Pyruvate decarboxylase (PDC; EC 4.1.1.1) catalyses the non-oxidative decarboxylation of pyruvate to acetaldehyde with the release of carbon dioxide, and is a key enzyme in homofermentative metabolism, where ethanol is the main fermentation product. ZpPDC forms a tetramer from four identical subunits in a dimer-of-dimers fashion. Each monomer contains a pyrimidine-binding (PYR) domain, a regulatory (R) domain and a pyrophosphate-binding (PP) domain. The TPP molecules bind across both subunits in each dimer, with the pyrophosphate group binding to the PP domain from one subunit and the pyrimidine ring binding to the PYR domain from the second subunit, thus forming two active sites in the dimer.

In this study, we present the crystal structure of recombinant ZpPDC at 2.15 Å resolution together with a comparison to the other known bacterial PDCs, thereby increasing the structural information available on these rare enzymes. The final model contains six tetramers in the asymmetric unit, each with a surface area of 65 000 Å2. It comprises 24 amino-acid chains of 555 amino acids, each with a TPP and a Mg2+ ion, and 4147 water molecules. Despite crystallization in the presence of pyruvate, no pyruvate molecules were visible anywhere in the structure, probably owing to catalytic turnover of the substrate to acetaldehyde and subsequent loss of this volatile product. However, six 1,2-ethanediol (EDO) molecules (the PEG monomer) are present, four of which can be found in the active sites in chains I, N, Q and R. Through pseudo-222 symmetry, the four monomers in a tetramer create four cofactor- and substrate-binding sites located in narrow clefts on the interfaces between the PYR domain of one monomer and the PP domain of a second monomer. The TPP molecule binds as indicated by the domain nomenclature, with the pyrophosphate group binding to the PP domain of one monomer and the pyrimidine ring binding to the PYR domain of a second monomer in the dimer. The pyrophosphate group of TPP is anchored to the protein by a Mg2+ ion. It forms an octahedral coordination sphere with the two O atoms on the diphosphate group of the TPP, the side-chain O atoms of Asp435 and Asn462, the main-chain O atom of Gly464 and a water molecule. Glu468 and Tyr289 from one monomer and Asp26, His112 and His113 from a second monomer interact with EDO through an extensive hydrogen-bond network.

>MYTVGMYLAERLAQIGLKHHFAVAGDYNLVLLDQLLLNKDMEQVYCCNELNCGFSAEGYARARGAAAAIVTFSVGAISAMNAIGGAYAENLPVILISGSPNTNDYGTGHILHHTIGTTDYNYQLEMVKHVTCAAESIVSAEEAPAKIDHVIRTALRERKPAYLEIACNVAGAECVRPGPINSLLRELEVDQTSVTAAVDAAVEWLQDRQNVVMLVGSKLRAAAAEKQAVALADRLGCAVTIMAAAKGFFPEDHPNFRGLYWGEVSSEGAQELVENADAILCLAPVFNDYATVGWNSWPKGDNVMVMDTDRVTFAGQSFEGLSLSTFAAALAEKAPSRPATTQGTQAPVLGIEAAEPNAPLTNDEMTRQIQSLITSDTTLTAETGDSWFNASRMPIPGGARVELEMQWGHIGWSVPSAFGNAVGSPERRHIMMVGDGSFQLTAQEVAQMIRYEIPVIIFLINNRGYVIEIAIHDGPYNYIKNWNYAGLIDVFNDEDGHGLGLKASTGAELEGAIKKALDNRRGPTLIECNIAQDDCTETLIAWGKRVAATNSRKPQALVPRGSGGGLEHHHHHH[24x]> MEEVEEFKYEPKSVKEIFIEMKDTVELMVDLAYASLLFGDKEIAEEVLELEERIDLLNYQLMMHSVLAARNVKEAEQVITILQIANAIEDISNAAGDLAKMVLEGVELHPVIKETILEGEEIIGKIQVYPESVIVGKTLGELDLATNTGVWIIAVRRGKRWIFGPNENFKIRAGDVLIGRGTRTSIDHLKEIARGAIRVIG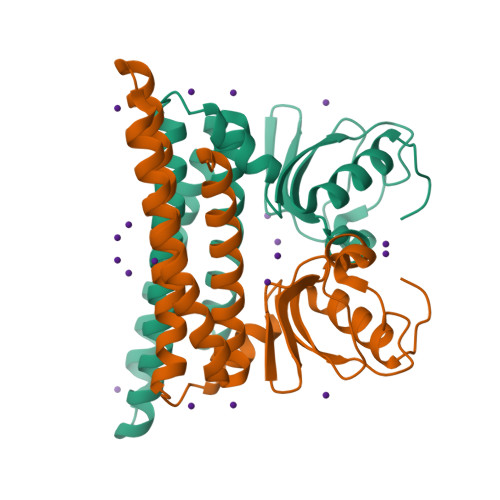NERA> MGSSHHHHHHSSGLVPRGSTSEVIEDEKQFYSKAKTYWKQIPPTVDGMLGGYGHISSIDINSSRKFLQRFLREGPNKTGTSCALDCGAGIGRITKRLLLPLFREVDM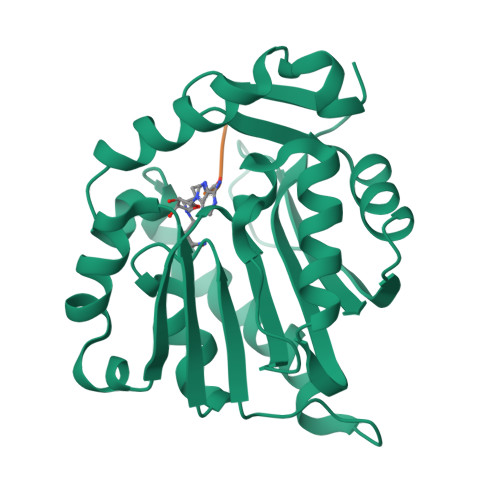VDITEDFLVQAKTYLGEEGKRVRNYFCCGLQDFTPEPDSYDVIWIQWVIGHLTDQHLAEFLRRCKGSLRPNGIIVIKDNMAQEGVILDDVDSSVCRDLDVVRRIICSAGLSLLAEERQENLPDEIYHVYSFALR> ATTLYENKTGTEDGYDYELWKDSGNTSMILNGGGTFSCQWSNINNCLFRKGKKFGGNQSYQQIGNISFDYGCDYHPNGNSYL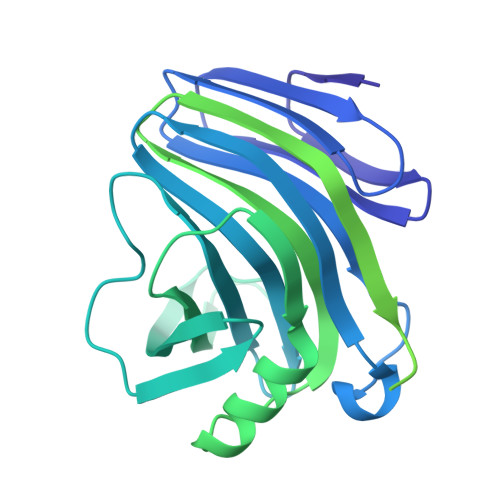CVYGWTTSPLVEFYIVDSWGSWRPPGGSPKGQIYVDGGTYDVYETTRVNQPSIQGNTTFQQYFSVRTERRTSGTINVTEHFKAWERMGMRMGNIYEAALNVEGYQSSGSANVYKNNMTIGGSSGQSGNQGGNQGGNQGGNQGGNTGSQTSGNETIVQCESMTKGGQYTGNINNPFGGVALYGNNDKVSYTQYFASGTHDFTLRGCSNNDNMARVDLKIGGETKGTFYYGGSYPAEYTIKNVNHGTGNQTIELVVTADNGQWDANIDYLKIGGAGVGGNESSGGNQGGNEGNQGGNAGNEGGNQAGNTGNQGGNEGNAGGQAQSGDNIVQCESMSKAGQYTGNINNPFDHHHHHH> MFVSDFRKEFYEVVQSQRVLLFVASDVDALCACKILQALFQCDHVQYTLVPVSGWQELETAFLEHKEQFHYFILINCGANVDLLDILQPDEDTIFFVCDTHRPVNVVNVYNDTQIKLLIKQDDDLEVPAYEDIFRDEEEDEEHSGNDSDGSEPVEQTMRRRQRREWEARRRDILFDYEQYEYHGTSSAMVMFELAWMLSKDLNDMLWWAIVGLTDQWVQDKITQMKYVTDVGVLQRHVSRHNHRNEDEENTLSVDCTRISFEYDLRLVLYQHWSLHDSLCNTSYTAARFKLWSVH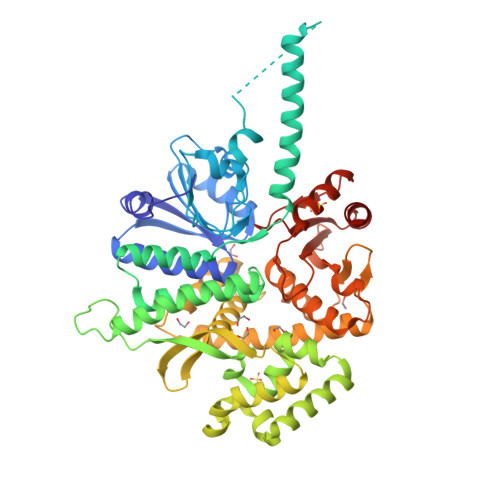GQKRLQEFLADMGLPLKQVKQKFQAMDISLKENLREMIEESANKFGMKDMRVQTFSIHFGFKHKFLASDVVFATMSLMESPEKDGSGTDHFIQALDSLSRSNLDKLYHGLELAKKQLRATQQTIASCLCTNLVISQGPFLYCSLMEGTPDVMLFSRPASLSLLSKHLLKSFVCSTKNRRCKLLPLVMAAPLSMEHGTVTVVGIPPETDSSDRKNFFGRAFEKAAESTSSRMLHNHFDLSVIELKAEDRSKFLDALISLLS>MNITKPFPLPTGYFGIPLGLAALSLAWFHLENLFPAARMVSDVLGIVASAVWILFILMYAYKLRYYFEEVRAEYH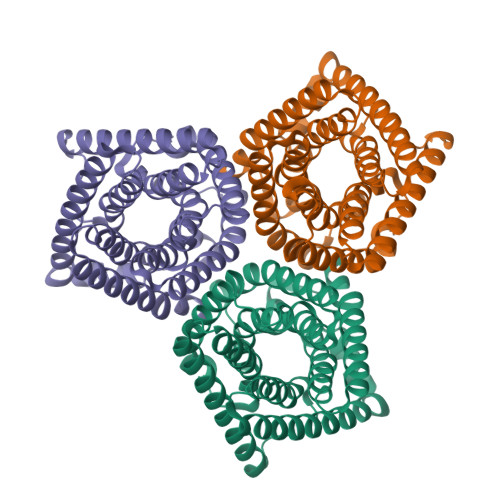SPVRFSFIALIPITTMLVGDILYRWNPLIAEVLIWIGTIGQLLFSTLRVSELWQGGVFEQKSTHPSFYLPAVAANFTSASSLALLGYHDLGYLFFGAGMIAWIIFEPVLLQHLRISSLEPQFRATMGIVLAPAFVCVSAYLSINHGEVDTLAKILWGYGFLQLFFLLRLFPWIVEKGLNIGLWAFSFGLASMANSATAFYHGNVLQGVSIFAFVFSNVMIGLLVLMTIYKLTKGQFFLK[3x]(2~{S})-~{N}2-[2-(4-methoxyphenyl)ethyl]-~{N}1-(naphthalen-1-ylmethyl)pyrrolidine-1,2-dicarboxamide 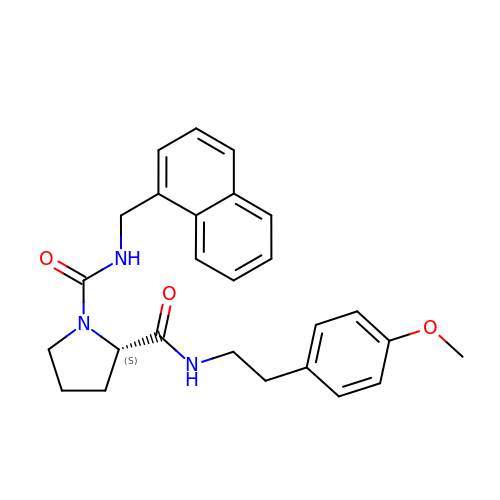| C26 H29 N3 O3 | HMNBKWNEJGMBRQ-DEOSSOPVSA-N biphenyl-4-ylacetic acid | C14 H12 O2 | 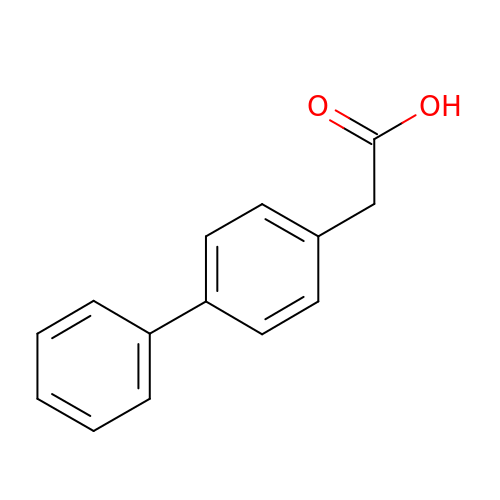QRZAKQDHEVVFRX-UHFFFAOYSA-N> SAPSVKGVSFDQANNLLIEPARIEEEELTLTILRQTGGLGISIAGGKGSTPYKGDDEGIFISRVSEEGPAARAGVRVGDKLLEVNGVALQGAEHHEAVEALRGAGTAVQMRVWRERM;> K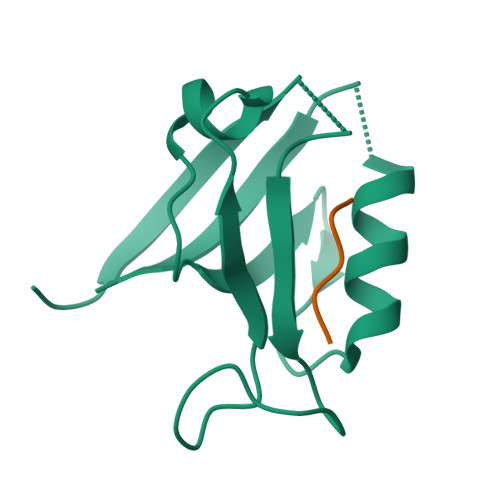MARTIESKV>MSIEKIWAREILDSRGNPTVEVDLYTAKGLFRAAVPSGASTGIYEALELRDGDKQRYLGKGVLKAVDHINSTIAPALISSGLSVVEQEKLDNLMLELDGTENKSKFGANAILGVSLAVCKAGAAERELPLYRHIAQLAGNSDLILPVPAFNVINGGSHAGNKLAMQEFMILPVGAESFRDAMRLGAEVYHTLKGVIKDKYGKDATNVGDEGGFAPNILENSEALELVKEAIDKAGYTEKIVIGMDVAASEFYRDGKYDLDFKSPTDPSRYITGDQLGALYQDFVRDYPVVSIE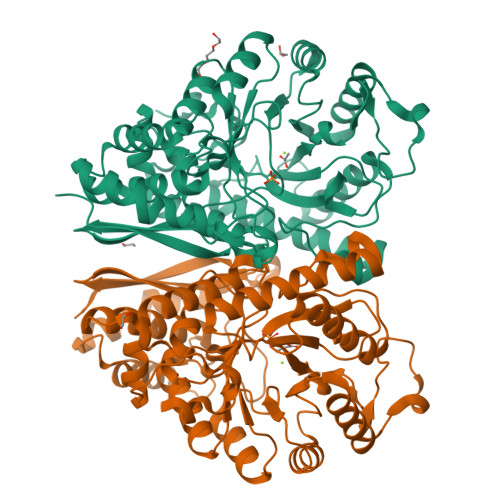DPFDQDDWAAWSKFTANVGIQIVGDDLTVTNPKRIERAVEEKACNCLLLKVNQIGSVTEAIQACKLAQENGWGVMVSHRSGETEDTFIADLVVGLCTGQIKTGAPCRSERLAKYNQLMRIEEELGDEARFAGHNFRNPSVLHHHHHH[2x]beta-L-fructofuranose | C6 H12 O6 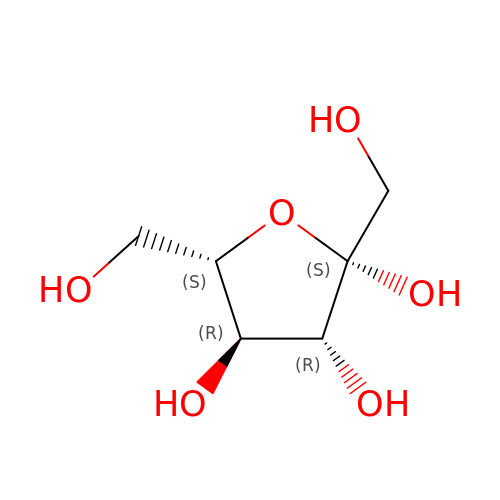| RFSUNEUAIZKAJO-AZGQCCRYSA-N[(2~{R},3~{S},4~{R},5~{R})-5-(6-aminopurin-9-yl)-3,4-bis(oxidanyl)oxolan-2-yl]methyl 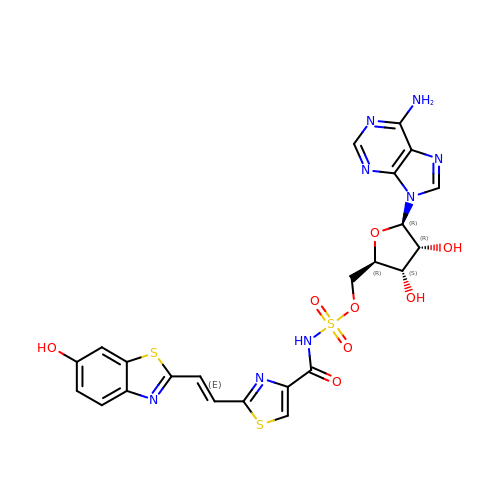~{N}-[[2-[(~{E})-2-(6-oxidanyl-1,3-benzothiazol-2-yl)ethenyl]-1,3-thiazol-4-yl]carbonyl]sulfamate | C23 H20 N8 O8 S3 | JXXQGJFRVFVJAK-AWGXURSZSA-N> HHHHMPVFHTRTIESILEPVAQQISHLVIMHEEGEVDGKAIPDLTAPVAAVQAAVSNLVRVGKETVQTTEDQILKRDMPPAFIKVENACTKLVQAAQMLQSDPYSVPARDYLIDGSRGILSGTSDLLLTFDEAEVRKIIRVCKGILEYLTVAEVVETMEDLVTYTKNLGPGMTKMAKMIDERQQELTHQEHRVMLVNSMNTVKELLPVLISAMKIFVTTKNSKNQGIEEALKNRNFTVEKMSAEINEIIR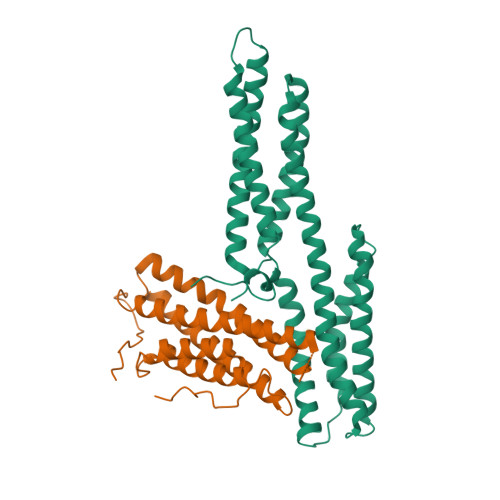VLQLTSWDEDAW;> DEEFPEQKAGEVINQPMMMAARQLHDEARKWSSKGNDIIAAAKRMALLMAEMSRLVRGGSGTKRALIQCAKDIAKASDEVTRLAKEVAKQCTDKRIRTNLLQVCERIPTISTQLKILSTVKATMLGRTNISDEESEQATEMLVHNAQNLMQSVKETVREAEAASIKIRTDAGFTLRWVRKTPWYQ> MSALYFQNLPSRPANKENYTRLLLKHINPNNKYAINPSLPLPHNKLQISSQPLMLLDDQMGLLEVSISRSSKMTNQAFLTFVTQEEADRFLEKYTTTALKVQGRKVRMGKARTNSLLGLSIEMQKKKGNDETYNLDIKKVLKARKLKRKLRSDDICAKKFRLKRQIRRLKHKLRSRKVEEAEIDRIVKEFETRRLENMKSQQENLKQSQKPLKRAKVSNTMENPPNKVLLIQNLPSGTTEQLLSQILGNEALVEIRLVSVRNLAFVEYETVADATKIKNQLGSTYKLQNNDVTIGFAK;> MNYNLSKYPDDVSRLFKPRPPLSYKRPTDYPYAKRQTNPNITGVANLLSTSLKHYMEEFPEGSPNNHLQRYEDIKLSKIKNAQLLDRRLQNWNPNVDPHIKDTDPYRTIFIGRLPYDLDEIELQKYFVKFGEIEKIRIVKDKITQKSKGYAFIVFKDPISSKMAFKEIGVHRGIQIKDRICIVDIERGRTVKYFKPRRLGGGLGGRGYSNRDSRLPGRFASASTSNPAERNYAPRLPRRETSSSAYSADRYGSSTLDARYRGNRPLLSAATPTAAVTSVYKSRNSRTRESQPAPKEAPDY;> MTRYYCEYCHSYLTHDTLSVRKSHLVGKNHLRITADYYRNKARDIINKHNHKRRHIGKRGRKERENSSQNETLKVTCLSNKEKRHIMHVKKMNQKELAQTSIDTLKLLYDGSPGYSKVFVDANRFDIGDLVKASKLPQRANEKSAHHSFKQTSRSRDETCESNPFPRLNNPKKLEPPKILSQWSNTIPKTSIFYSVDILQTTIKESKKRMHSDGIRKPSSANGYKRRRYGN;> MPDETNFTIEDIEPRPDALRGLDTQFLQDNTALVQAYRGLDWSDISSLTQMVDVIEQTVVKYGNPNDSIKLALETILWQILRKYPLLFGFWKRFATIEYQLFGLKKSIAVLATSVKWFPTSLELWCDYLNVLCVNNPNETDFIRNNFEIAKDLIGKQFLSHPFWDKFIEFEVGQKNWHNVQRIYEYIIEVPLHQYARFFTSYKKFLNEKNLKTTRNIDIVLRKTQTTVNEIWQFESKIKQPFFNLGQVLNDDLENWSRYLKFVTDPSKSLDKEFVMSVFDRCLIPCLYHENTWMMYIKWLTKKNISDEVVVDIYQKANTFLPLDFKTLRYDFLRFLKRKYRSNNTLFNNIFNETVSRYLKIWPNDILLMTEYLCMLKRHSFKNSLDQSPKEILEKQTSFTKILETSITNYINNQIDAKVHLQTLINDKNLSIVVVELIKTTWLVLKNNMQTRKYFNLYQKNILIKNSVPFWLTYYKFEKSNVNFTKLNKFIRELGVEIYLPTTVMNDILTDYKTFYLTHSNIVTYESSIIDSNTFDPILYPELKMSNPKYDPVLNTTANVDWHKKTEWKEAGHIGITTERPQISNSIIECNSGTLIQKPISLPNFRNLEKINQVKINDLYTEEFLKEGK;> MDKYTALIHDENFSTLTLNVSRYPKSLAYWEKLLNYIVKASAPICKSTEPQLLKLIRCTYSSMLNEFPYLENYYIDFALLEYKLGNVSMSHKIFQRGLQAFNQRSLLLWTSYLKFCNNVISHQKQLFKKYETAEEYVGLHFFSGEFWDLYLEQISSRCTSSKKYWNVLRKILEIPLHSFSKFYALWLQRIDDIMDLKQLSQLTSKDELLKKLKIDINYSGRKGPYLQDAKKKLKKITKEMYMVVQYQVLEIYSIFESKIYINYYTSPETLVSSDEIETWIKYLDYTITLQTDSLTHLNFQRALLPLAHYDLVWIKYSKWLINSKNDLLGAKNVLLMGLKFSLKKTEIIKLLYSVICKLNEYVLLRNLLEKIESSYSDNVENVDDFEIFWDYLQFKTFCQNSLYSSRYSDSQSNGLLNKELFDKVWKRLSCKEKKSGQEILLNNLVQFYSKDTVEFVEKNIFQKIIEFGWEYYLQNGMFWNCYCRLIYFDTSRSYLDKRQYIVRKIWPQIDKKFAQSVLPSLTEFCESYFPEEMDTLEEMFTEEP;> MSYKQTTYYPSRGNLVRNDSSPYTNTISSETNNSSTSVLSLQGASNVSLGTTGNQLYMGDLDPTWDKNTVRQIWASLGEANINVRMMWNNTLNNGSRSSMGPKNNQGYCFVDFPSSTHAANALLKNGMLIPNFPNKKLKLNWATSSYSNSNNSLNNVKSGNNCSIFVGDLAPNVTESQLFELFINRYASTSHAKIVHDQVTGMSKGYGFVKFTNSDEQQLALSEMQGVFLNGRAIKVGPTSGQQQHVSGNNDYNRSSSSLNNENVDSRFLSKGQSFLSNGNNNMGFKRNHMSQFIYPVQQQPSLNHFTDPNNTTVFIGGLSSLVTEDELRAYFQPFGTIVYVKIPVGKCCGFVQYVDRLSAEAAIAGMQGFPIANSRVRLSWGRSAKQTALLQQAMLSNSLQVQQQQPGLQQPNYGYIPSSTCEAPVLPDNNVSSTMLPGCQILNYSNPYANANGLGSNNFSFYSNNNATNTQATSLLADTSSMDLSGTGGQQVIMQGSEAVVNSTNAMLNRLEQGSNGFMFA;> MRPRRRGLAYHHTKPKGQLSQGHYPTTSNDGQRRKVGNSEAFQSFDIWKNLDRIRSTKKNAGQFIKGSLLILPMRTEDKQQFDECMDELHKYISKDILRCYPQKEQKDEGMLFYIVLKDFNILDSCFVLSVLLAFQKRLWMAPSEKSYFRVPKNINLTGSFYLPKNIETGRGHIITSYRREQPSSSIVEVGFNVVPDFQQFQVKACHVSKFMNELSNFFSQVEFGKCEANVINYFKREYNRTYSQISLALYELPLIGDGLFDIKSYISKTRPIIETSKAQMIKHISEMKAYNEISGLQGDQFPRQQRPLSNSPSSNSISSSQTIEAGATSYQTQPQRHAVNKPSNVLNSSNRHSGPKTFEDGRYSEGNKPGFMTQDEIKQHCIGTIKASMDAVKKKSSYQILKTYVRCPRQNYIDIVYQNLNDLRSKTNCNIVVLNLNNLHESQMWLESLNTTNYTIFAQAPHPSTIRVISIGGVGEYIVKALELILNILEH;> MSTMSTPAAEQRKLVEQLMGRDFSFRHNRYSHQKRDLGLHDPKICKSYLVGECPYDLFQGTKQSLGKCPQMHLTKHKIQYEREVKQGKTFPEFEREYLAILSRFVNECNGQISVALQNLKHTAEERMKIQQVTEELDVLDVRIGLMGQEIDSLIRADEVSMGMLQSVKLQELISKRKEVAKRVRNITENVGQSAQQKLQVCEVCGAYLSRLDTDRRLADHFLGKIHLGYVKMREDYDRLMKNNRTTNASKTATTLPGRRFV;> MRDIVFVSPQLYLSSQEGWKSDSAKSGFIPILKNDLQRFQDSLKHIVDARNSLSETLLNSNDDGSIHNSDQNTGLNKDKEASIADNNSANKCATSSSRYQELKQFLPISLDQQIHTVSLQGVSSSFSRGQIESLLDHCLNLALTETQSNSALKVEAWSSFSSFLDTQDIFIRFSKVDEDEAFVNTLNYCKALFAFIRKLHEDFKIELHLDLNTKEYVEDRTGTIPSVKPEKASEFYSVFKNIEDQTDERNSKKEQLDDSSTQYKVDTNTLSDLPSDALDQLCKDIIEFRTKVVSIEKEKKMKSTYEESRRQRHQMQKVFDQIRKNHSGAKGSANTEEEDTNMEDEDEEDDTEDDLALEKRKEERDLEESNRRYEDMLHQLHSNTEPKIKSIRADIMSAENYEEHLEKNRSLYLKELLHLANDVHYDHHRSFKEQEERRDEEDRAKNGNAKELAPIQLSDGKAISAGKAAAITLPEGTVKSENYNADKNVSESSEHVKIKFDFKKAIDHSVESSSEDEGYRESELPPTKPSERSAAEDRLPFTADELNIRLTNLKESRYVDELVREFLGVYEDELVEYILENIRVNQSKQALLNELRETFDEDGETIADRLWSRKEFRLGT;> MSIWKEAKDASGRIYYYNTLTKKSTWEKPKELISQEELLLRENGWKAAKTADGKVYYYNPTTRETSWTIPAFEKKVEPIAEQKHDTVSHAQVNGNRIALTAGEKQEPGRTINEEESQYANNSKLLNVRRRTKEEAEKEFITMLKENQVDSTWSFSRIISELGTRDPRYWMVDDDPLWKKEMFEKYLSNRSADQLLKEHNETSKFKEAFQKMLQNNSHIKYYTRWPTAKRLIADEPIYKHSVVNEKTKRQTFQDYIDTLIDTQKESKKKLKTQALKELREYLNGIITTSSSETFITWQQLLNHYVFDKSKRYMANRHFKVLTHEDVLNEYLKIVNTIENDLQNKLNELRLRNYTRDRIARDNFKSLLREVPIKIKANTRWSDIYPHIKSDPRFLHMLGRNGSSCLDLFLDFVDEQRMYIFAQRSIAQQTLIDQNFEWNDADSDEITKQNIEKVLENDRKFDKVDKEDISLIVDGLIKQRNEKIQQKLQNERRILEQKKHYFWLLLQRTYTKTGKPKPSTWDLASKELGESLEYKALGDEDNIRRQIFEDFKPESSAPTAESATANLTLTASKKRHLTPAVELDY;> MSHPIQFVNANNSDKSHQLGGQYSIPQDLRENLQKEAARIGENEKDVLQEKMETRTVQNREDSYHKRRFDMKFEPDSDTQTVTSSENTQDAVVPRKRKSRWDVKGYEPPDESSTAVKENSDSALVNVEGIHDLMFFKPSDHKYFADVISKKPIDELNKDEKKERTLSMLLLKIKNGNTASRRTSMRILTDKAVTFGPEMIFNRLLPILLDRSLEDQERHLMIKTIDRVLYQLGDLTKPYVHKILVVAAPLLIDEDPMVRSTGQEIITNLSTVAGLKTILTVMRPDIENEDEYVRNVTSRAAAVVAKALGVNQLLPFINAACHSRKSWKARHTGIKIVQQIGILLGIGVLNHLTGLMSCIKDCLMDDHVPVRIVTAHTLSTLAENSYPYGIEVFNVVLEPLWKGIRSHRGKVLSSFLKAVGSMIPLMDPEYAGYYTTEAMRIIRREFDSPDDEMKKTILLVLQKCSAVESITPKFLREEIAPEFFQKFWVRRVALDRPLNKVVTYTTVTLAKKLGCSYTIDKLLTPLRDEAEPFRTMAVHAVTRTVNLLGTADLDERLETRLIDALLIAFQEQTNSDSIIFKGFGAVTVSLDIRMKPFLAPIVSTILNHLKHKTPLVRQHAADLCAILIPVIKNCHEFEMLNKLNIILYESLGEVYPEVLGSIINAMYCITSVMDLDKLQPPINQILPTLTPILRNKHRKVEVNTIKFVGLIGKLAPTYAPPKEWMRICFELLELLKSTNKEIRRSANATFGFIAEAIGPHDVLVALLNNLKVQERQLRVCTAVAIGIVAKVCGPYNVLPVIMNEYTTPETNVQNGVLKAMSFMFEYIGNMSKDYIYFITPLLEDALTDRDLVHRQTASNVITHLALNCSGTGHEDAFIHLMNLLIPNIFETSPHAIMRILEGLEALSQALGPGLFMNYIWAGLFHPAKNVRKAFWRVYNNMYVMYQDAMVPFYPVTPDNNEEYIEELDLVL;> MWGGGKMAVVSLSPHTAKMRKLFGQASTTMAYDGLKREAERRTRSDHNITMVAKDDELYLYHLTLKKQTNFVHSCIGHFVDLEAGSKREQSQLCVATETHLELYDTADGELKLIAKFQNLFATITSMKSLDLPHSGSRAKASNWPTFLALTSDSGNLSIVQIIMHAGALRLKTLVNQPLTRTTLRRVSPISYMEIDPNGRCIILSSVEQNKLCFLVDYAQKLRISSPLEIIRPHMVTLDMAVVDVNFNNPCFVTLEIDNAATQLSVHLIFYVLELGLNHIVKKADYLVNPSANFVLSLPDLSRYNITTSLSDNNYDADYDTLFNPFVVIGFENHILVKDMNGFFSLKVEIPKRSITNSRHKNVTIISGIVQKLKNDFFVLLQSNHGDLFKLTVSPDTNDRNRPLVQLSYFDTIQNSHQLHIFKNGYLFALSEMNNNFLFQFEKLGVEKNDFSNVLTSKDPNKSLVFEPSIKLQNLSILSQQLNLNPSIKSQIVSDSPLSIATKHFTNNKIITLTNAVNYSNLISTSLPPNATKLWLIPDPATTGDNNTLLFITFPKKTMILQIDNESMEELTPDEATRSAFKLSQDTTIHTCLMGSHSIIQVCTAELRHIVPTGKSRYSNKLTWVPPAGIRIVCATSSKTQLIISLSNYELVYFKIDVSSDSLIELTTHPELDTMPSKVAIVQDTQHADLLAIADNEGMIKIMSLKDQKEDFLTVISLQLVSEKISDMIMVRDSSIGQLNLHVGLENGVYMKFHIGDVDGSFTDIKRRFLGLKPVSLSYLREISVSLNNEEEEEEEEDDDDEKEEEEINSSGAKWMSCVVCHSSSTWVSYTWKNVWTIRQLKDQNMLSCSKFVNADVAINGVCSISSSGRLNIGRVSNFPTLDNWFHVHESSVNKQENGGGDESNEEEEDEMEEEMEMLQISTFRPRTILSFPNNPKSILFIDNHSGKKQCRISLQIDGECLKFGSSDHLYKILDDIDCVSAAIIDFTRQADHLIICAGDKRLLTYKILVNKDKLSFDIELLHQTEIISPIHAMLKFKNFLLTAMGSTIVLYGLGKKQLLRRSVTQTPVSITKIVSMHQWNYERLAVGDIHESVTLFIWDPAGNVFIPYVDDSVKRHVTVLKFLDEATVIGADRYGNAWTLRSPPECEKIMSNHDPSELSNGAIKYPLDVITLQQKLPNTYDCKFKFQLLNHFFVNDIITDFHILDSLSNSDRPGCIYMGLQGTVGCFIPLLSKGNVFMMGNIENIMAEADDTFYLDYESRKKNNNMRKEDDEEESGSVVLQGRHGIEDEIICEGSCSILGRDHQEYRSYYAPVRKVIDGDLCENFLRLSLNEQEFLAKNLKSVQVEDIIQTINEVRTNYM;> MARTKSRKRSGNNQNKNASVVNNKAEIAAMIDARRLEQKKKGGVTNSKGKTNKVVDAKLEKEFKDVLQRFQVQENDTPKEITKDEKNNHVVIVEKNPVMNRKHTAEDELEDTPSDGIEEHLSARKRRKTEKPSLSQLKSQVPYPQIIEWYDCDARYPGLLASIKCTKNVIPVPSHWQSKKEYLSGRSLLGKRPFELPDIIKKTNIEQMRSTLPQSGLDGQDEKSLKEASRARVQPKMGALDLDYKKLHDVFFKIGANWKPDHLLCFGDVYYENRNLFEETNWKRMVDHKRPGRISQELRAIMNLPEGQLPPWCMKMKDIGLPTGYPDLKIAGLNWDITNLKGDVYGKIIPNHHSRSKKQGRNYFGALISFETPEFENSKEDTQANAENGRQDDKIDDEVEHKLDHFQEDISEVTSAEEKLERNEEESEKQLYTVLK;> MNYSADSGNTVYVGNIDPRITKEQLYELFIQINPVLRIKYPKDKVLQAYQGYAFIEFYNQGDAQYAIKIMNNTVRLYDRLIKVRQVTNSTGTTNLPSNISKDMILPIAKLFIKNLADSIDSDQLVKIFNKFGKLIREPEIFYLSNGKLKCAYVYFEDFEKADLAIKSLNNQLVANNRITVDYAFKENGKGNAKYGDDVDRLLNKEALKHNMLK;> MSRHQFDLIMCLKQPGVQTGLLCEKCDGKCPICDSYVRPKRKVRVCENCSFGKQAKNCIICNLNVGVNDAFYCWECCRLGKDKDGCPRILNLGSNRLDRHFEKKKKV;> MNLLETRRSLLEEMEIIENAIAERIQRNPELYYHYIQESSKVFPDTKLPRSSLIAENKIYKFKKVKRKRKQIILQQHEINIFLRDYQEKQQTFNKINRPEETQEDDKDLPNFERKLQQLEKELKNEDENFELDINSKKDKYALFSSSSDPSRRTNILSDRARDLDLNEIFTRDEQYGEYMELEQFHSLWLNVIKRGDCSLLQFLDILELFLDDEKYLLTPPMDRKNDRYMAFLLKLSKYVETFFFKSYALLDAAAVENLIKSDFEHSYCRGSLRSEAKGIYCPFCSRWFKTSSVFESHLVGKIHKKNESKRRNFVYSEYKLHRYLKYLNDEFSRTRSFVERKLAFTANERMAEMDILTQKYEAPAYDSTEKEGAEQVDGEQRDGQLQEEHLSGKSFDMPLGPDGLPMPYWLYKLHGLDREYRCEICSNKVYNGRRTFERHFNEERHIYHLRCLGIEPSSVFKGITKIKEAQELWKNMQGQSQLTSIAAVPPKPNPSQLKVPTELELEEEDEEGNVMSKKVYDELKKQGLV;> MNYLEGVGSKKGGGGIASESQFNLQRRKEVESLLSKGENVPYTFQDEKDDQVRSNPYIYKNHSGKLVCKLCNTMHMSWSSVERHLGGKKHGLNVLRRGISIEKSSLGREGQTTHDFRQQQKXXXXXXXXXXXXXXXXIIEAKQSLKNNGTIPVCKIATVKNPKNGSVGLAIQVNYSSEVKENSVDSDDKAKVPPLIRIVSGLELSDTKQKGKKFLVIAYEPFENIAIELPPNEILFSENNDMDNNNDGVDELNKKCTFWDAISKLYYVQFFFKQAEQEQADV;> MEPEDTQLKEDIKTTVNYIKQHGVEFENKLLEDERFSFIKKDDPLHEYYTKLMNEPTDTVSGEDNDRKSEREIARPPDFLFSQYDTGISRRDMEVIKLTARYYAKDKSIVEQMISKDGEARLNFMNSSHPLHKTFTDFVAQYKRVYSFTGQEIKKSKRTILDNCFERTQYWEFEKDKDREHDKLVELCKIQFAAIPWDKFTQVAKFSIPEDTEIFEGSLDLEQMRLRRVQTGIKLFDSIKPTNEEEKIVSDQGKQKGGDSKGKKRKIRAVGETRLKKSKK;> MKFTPSIVIDAPQYYVDHFNGKYNVDKCVILRDLQLETDSESMPSSLKHLTKPTHILDLTNNDLIMIPDLSRRDDIHTLLLGRNNIVEVDGRLLPMNVQNLTLSNNSIRRFEDLQRLRRAPRTLKNLTLIGNQVCHLANYREHVLRLVPHLETLDFQNVTAEERKSAMSFPRQADGDTLGPVNTAIRDNGSRDKTMEIMNLVVSKMTVERRNELKKQLAEATSLEEIARLEKLLSGGV;> MVEPARKKQRIDRDTHHTVAEPVTEAKNTLYVSQLNEKINMQRLRVNLFLLFATFGEVLKVSMNFKKQRGQAFITMRTIDQASLAQISLNGERFFGKPLKVEFSKSETKTL;> MAEKQRQLKLQKIYKQKYIGLGDESTTREQWQRNVRNDTLNTLQGHSASLEYVSLSRGDLSIRDTRIHLLKSMSPGYKAYLREER;>MSKIQVAHSSRLANLIDYKLRVLTQDGRVYIGQLMAFDKHMNLVLNECIEERVPKTQLDKLRPRKDSKDGTTLNIKVEKRVLGLTILRGEQILSTVVEDKPLLSKKERLVRDKKEKKQAQKQTKLRKEKEKKPGKIAKPNTANAKHTSSNSREIAQPSSSRYNGGNDNIGANRSRFNNEAPPQTRKFQPPPGFKRK[2x];>MTMNGIPVKLLNEAQGH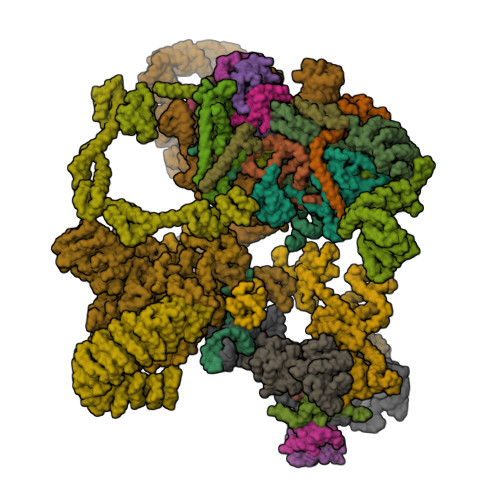IVSLELTTGATYRGKLVESEDSMNVQLRDVIATEPQGAVTHMDQIFVRGSQIKFIVVPDLLKNAPLFKKNSSRPMPPIRGPKRR[2x];>[2x]MSNKVKTKAMVPPINCIFNFLQQQTPVTIWLFEQIGIRIKGKIVGFDEFMNVVIDEAVEIPVNSADGKEDVEKGTPLGKILLKGDNITLITSAD;>[2x]MSESSDISAMQPVNPKPFLKGLVNHRVGVKLKFNSTEYRGTLVSTDNYFNLQLNEAEEFVAGVSHGTLGEIFIRCNNVLYIRELPN;>[2x]MVSTPELKKYMDKKILLNINGSRKVAGILRGYDIFLNVVLDDAMEINGEDPANNHQLGLQTVIRGNSIISLEALDAI;>[2x]MKLVNFLKKLRNEQVTIELKNGTTVWGTLQSVSPQMNAILTDVKLTLPQPRLNKLNSNGIAMASLYLTGGQQPTASDNIASLQYINIRGNTIRQIILPDSLNLDSLLVDQKQLNSLRRSGQIANDPSKKRRRDFGAPANKRPRRGL;>[2x]MSSQIIDRPKHELSRAELEELEEFEFKHGPMSLINDAMVTRTPVIISLRNNHKIIARVKAFDRHCNMVLENVKELWTEKKGKNVINRERFISKLFLRGDSVIVVLKTPVE;> METIDSKQNINRESLLEERRKKLAKWKQKKAQFDAQKEHQTSRNDIVTNSLEGKQTTEKFTERQERVKEELRKRKNEFRKSDEPVSVKPSKKKSKRSKVKKKISFDFSDDDDSEIGVSFRSKEHIQKAPEHDNEKDPLDEFMTSLKEEKMSNSKGMYDRGDILDVEDQLFELGGTDDEDVEDNTDNSNIAKIAKLKAKKRVKQIYYSPEELEPFQKNFYIESETVSSMSEMEVEELRLSLDNIKIKGTGCPKPVTKWSQLGLSTDTMVLITEKLHFGSLTPIQSQALPAIMSGRDVIGISKTGSGKTISYLLPLLRQVKAQRPLSKHETGPMGLILAPTRELALQIHEEVTKFTEADTSIRSVCCTGGSEMKKQITDLKRGTEIVVATPGRFIDILTLNDGKLLSTKRITFVVMDEADRLFDLGFEPQITQIMKTVRPDKQCVLFSATFPNKLRSFAVRVLHSPISITINSKGMVNENVKQKFRICHSEDEKFDNLVQLIHERSEFFDEVQSENDGQSSDVEEVDAKAIIFVSSQNICDFISKKLLNAGIVTCAIHAGKPYQERLMNLEKFKREKNSILLCTEVLSRGLNVPEVSLVIIYNAVKTFAQYVHTTGRTARGSRSGTAITLLLHDELSGAYILSKAMRDEEIKALDPLQAKELQEMSAKFESGMKKGKFRLSKGFGGKGLENIKSKREEAQNKDLELKKNDKRSDDLEKKISNPREGHDSVSESSALIPRLNYELFKESTDGSIIFYAKVYINDLPQIVRWEATKNTTLLFIKHETGCSITNKGKFYPEGKEPKNENDEPKLYLLIEGQDEKDIQLSIELLEQKVKEGVVKAASLSLKSTKY> MSLRSGGRRRADPGADGEASRDDGATSSVSALKRLERSQWTDKMDLRFGFERLKEPGEKTGWLINMHPTEILDEDKRLGSAVDYYFIQDDGSRFKVALPYKPYFYIATRKGCEREVSSFLSKKFQGKIAKVETVPKEDLDLPNHLVGLKRNYIRLSFHTVEDLVKVRKEISPAVKKNREQDHASDAYTALLSSVLQRGGVITDEEETSKKIADQLDNIVDMREYDVPYHIRLSIDLKIHVAHWYNVRYRGNAFPVEITRRDDLVERPDPVVLAFAIATTKLPLKFPDAETDQIMMISYMIDGQGYLITNREIVSEDIEDFEFTPKPEYEGPFCVFNEPDEAHLIQRWFEHVQETKPTIMVTYNGDFFDWPFVEARAAVHGLSMQQEIGFQKDSQGEYKAPQCIHMDCLRWVKRDSYLPVGSHNLKAAAKAKLGYDPVELDPEDMCRMATEQPQTLATYSVSDAVATYYLYMKYVHPFIFALCTIIPMEPDEVLRKGSGTLCEALLMVQAFHANIIFPNKQEQEFNKLTDDGHVLDSETYVGGHVEALESGVFRSDIPCRFRMNPAAFDFLLQRVEKTLRHALEEEEKVPVEQVTNFEEVCDEIKSKLASLKDVPSRIECPLIYHLDVGAMYPNIILTNRLQPSAMVDEATCAACDFNKPGANCQRKMAWQWRGEFMPASRSEYHRIQHQLESEKFPPLFPEGPARAFHELSREEQAKYEKRRLADYCRKAYKKIHITKVEERLTTICQRENSFYVDTVRAFRDRRYEFKGLHKVWKKKLSAAVEVGDAAEVKRCKNMEVLYDSLQLAHKCILNSFYGYVMRKGARWYSMEMAGIVCFTGANIITQARELIEQIGRPLELDTDGIWCVLPNSFPENFVFKTTNVKKPKVTISYPGAMLNIMVKEGFTNDQYQELAEPSSLTYVTRSENSIFFEVDGPYLAMILPASKEEGKKLKKRYAVFNEDGSLAELKGFEVKRRGELQLIKIFQSSVFEAFLKGSTLEEVYGSVAKVADYWLDVLYSKAANMPDSELFELISENRSMSRKLEDYGEQKSTSISTAKRLAEFLGDQMVKDAGLSCRYIISRKPEGSPVTERAIPLAIFQAEPTVRKHFLRKWLKSSSLQDFDIRAILDWDYYIERLGSAIQKIITIPAALQQVKNPVPRVKHPDWLHKKLLEKNDVYKQKKISELFTLEGRRQVTMAEASEDSPRPSAPDMEDFGLVKLPHPAAPVTVKRKRVLWESQEESQDLTPTVPWQEILGQPPALGTSQEEWLVWLRFHKKKWQLQARQRLARRKRQRLESAEGVLRPGAIRDGPATGLGSFLRRTARSILDLPWQIVQISETSQAGLFRLWALVGSDLHCIRLSIPRVFYVNQRVAKAEEGASYRKVNRVLPRSNMVYNLYEYSVPEDMYQEHINEINAELSAPDIEGVYETQVPLLFRALVHLGCVCVVNKQLVRHLSGWEAETFALEHLEMRSLAQFSYLEPGSIRHIYLYHHAQAHKALFGIFIPSQRRASVFVLDTVRSNQMPSLGALYSAEHGLLLEKVGPELLPPPKHTFEVRAETDLKTICRAIQRFLLAYKEERRGPTLIAVQSSWELKRLASEIPVLEEFPLVPICVADKINYGVLDWQRHGARRMIRHYLNLDTCLSQAFEMSRYFHIPIGNLPEDISTFGSDLFFARHLQRHNHLLWLSPTARPDLGGKEADDNCLVMEFDDQATVEINSSGCYSTVCVELDLQNLAVNTILQSHHVNDMEGADSMGISFDVIQQASLEDMITGGQAASAPASYDETALCSNTFRILKSMVVGWVKEITQYHNIYADNQVMHFYRWLRSPSSLLHDPALHRTLHNMMKKLFLQLIAEFKRLGSSVIYANFNRIILCTKKRRVEDAIAYVEYITSSIHSKETFHSLTISFSRCWEFLLWMDPSNYGGIKGKVSSRIHCGLQDSQKAGGAEDEQENEDDEEERDGEEEEEAEESNVEDLLENNWNILQFLPQAASCQNYFLMIVSAYIVAVYHCMKDGLRRSAPGSTPVRRRGASQLSQEAEGAVGALPGMITFSQDYVANELTQSFFTITQKIQKKVTGSRNSTELSEMFPVLPGSHLLLNNPALEFIKYVCKVLSLDTNITNQVNKLNRDLLRLVDVGEFSEEAQFRDPCRSYVLPEVICRSCNFCRDLDLCKDSSFSEDGAVLPQWLCSNCQAPYDSSAIEMTLVEVLQKKLMAFTLQDLVCLKCRGVKETSMPVYCSCAGDFALTIHTQVFMEQIGIFRNIAQHYGMSYLLETLEWLLQKNPQLGH;>MFEARLVQGSILKKVLEALKDLINEACWDISSSGVNLQSMDSSHVSLVQLTLRSEGFDTYRCDRNLAMGVNLTSMSKILKCAGNEDIITLRAEDNADTLALVFEAPNQEKVSDYEMKLMDLDVEQLGIPEQEYSCVVKMPSGEFARICRDLSHIGDAVVISCAKDGVKFSASGELGNGNIKLSQTSNVDKEEEAVTIEMNEPVQLTFALRYLNFFTKATPLSSTVTLSMSADVPLVVEYKIADMGHLKYYLAPKIEDEEGS[3x]

In eukaryotes, the leading strand DNA is synthesized by Polε and the lagging strand by Polδ. These replicative polymerases have higher processivity when paired with the DNA clamp PCNA. Here we report two cryo-EM structures of human Polε–PCNA–DNA complex, one in an incoming nucleotide bound state and the other in a nucleotide exchange state. The structures reveal an unexpected three-point interface between the Polε catalytic domain and PCNA, with the conserved PIP (PCNA interacting peptide)-motif, the unique P-domain, and the thumb domain each interacting with a different protomer of the PCNA trimer.

In contrast, the ternary Polε–PCNA–DNA structure lacks the incoming dTTP and the finger domain is in an open position. We refer to this structure as the “nucleotide exchange state” because the Pol is open and poised to bind a new dNTP. The nucleotide exchange state is transient and dynamic, likely accounting for the medium resolution (5.01 Å) of the EM map. The ternary complex model was derived by rigidly-body fitting the quaternary model into the medium-resolution cryo-EM map. But the bound DNA is resolved with clear major and minor grooves features, and the modeled P/T DNA fits the EM density well. In the nucleotide exchange state, the finger domain is in an open position, and there is no incoming nucleotide in the Polε activate site. Superimposing this state with the above-described nucleotide bound state by the shared PCNA reveals that the finger domain rotates by 25° to close the activate site. Because the P-domain is elongated, and its [4Fe-4S] containing upper end is connected to the finger domain, a closer inspection reveals that the [4Fe-4S] containing tip of the P-domain functions as a hinge for finger rotation. The [4Fe-4S] cluster was previously shown to be essential to the yeast Polε function. This cluster likely plays a structural role to strengthen the hinge to support the finger rotation. Overall, the transition from the nucleotide exchange to nucleotide bound state moves the DNA down slightly to create an insertion site to accommodate the incoming nucleotide.>MAHHHHHHMISFYGYTHFDGRTLKNKYGMQGKALQERCAYDLLQAMLNLRKEPLPEKFDSSYLKYLHQRLYEKMFEWAGCTCDTPFTFSDGTVTKVPINNKIKEGLKRIDQILAEKNNFQGLSRKEFIHEVSTVFILLNKIRPFMVGNKYVQRIFFEQIAEAAGHKLDFSVVTEKRMQFAIHAALSFDGNNNRGNITPMLHLFEDISNPEKVGILKEFMIYI[6x]

Proteins containing a FIC domain catalyze AMPylation and other post-translational modifications (PTMs). Among these, Bartonella effector proteins (Beps) comprise a particularly diverse ensemble of FIC domains that subvert various host cellular functions. The FIC fold comprises eight conserved α-helices and encompasses a characteristic active site loop between helices α4 and α5 that forms most of the catalytic center and the substrate binding pocket. Additionally, FIC domains generally contain a β-hairpin between helix α2 and helix α3 that is referred to as the “flap” and mediates docking of a target segment in extended conformation via β-strand augmentation.

Members of the Bep5 sub-clade are characterized by the absence of the flap. Indeed, the structure of Bcl_Bep5 shows that the Bep element is directly followed by α3. The structurally required residues of the FIC signature motif (PFxx(N/S)G) are conserved, explaining the canonical fold of the FIC loop, but most other residues of the FIC signature motif are distinct. Bcl_Bep5 FIC crystals were grown from a solution of 20% w/v PEG 3350, 0.1 M sodium citrate/citric acid, pH 4.0, and 0.2 M sodium citrate tribasic. Data for Bqu_BepC FIC, B15_Bep8 FIC, and Bcl_Bep5 FIC were collected at 100 K on a Rayonix MX-300 detector at a wavelength of 0.9786 Å on beamline 21-ID-G at the Advanced Photon Source (APS, Argonne, IL, USA).>SPDKLKKVLDKLRLDPKDISEAAETVNKVVERLLRRMQKRESEFKGVEQLFVGSIYEKVKISAPNEFDVMFKLEVPRIELQEYYETGAFYLVKFKRIPRGNPLSHFLEGEVLSATKMLSKFR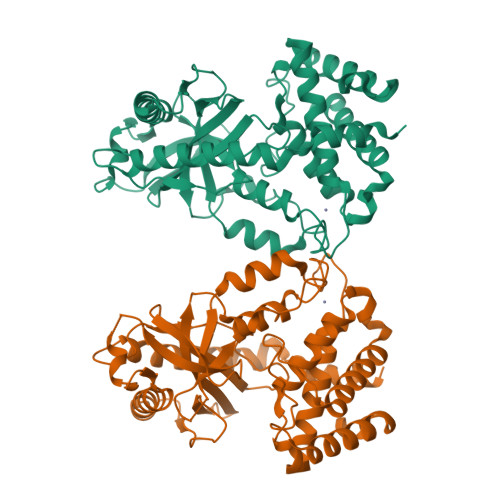KIIKEEVKEIKDIDVSVEKEKPGSPAVTLLIRNPEEISVDIILALESKGSWPISTKEGLPIQGWLGTKVRTNLRREPFYLVPKNAKDGNSFQGETWRLSFSHTEKYILNNHGIEKTCCESSGAKCCRMECLMLMKYLLEQLKKEFQELDAFCSYHVKTAIFHMWTQDPQDSQWDPRNLSSCFDKLLAFFLECLRTEKLDHYFIPKFNLFSQELIDRKSKEFLSKKIEYERNNGFPIFDKL[2x]> ELPQMTQQLNSDDMQEQLSATVKFRQILSREHRPPIDVVIQAGVVPRLVEFMRENQPEMLQLEAAWALTNIASGTSAQTKVVVDADAVPLFIQLLYTGSVEVKEQAIWALGNVAGDSTDYRDYVLQCNAMEPILGLFNSNKPSLIRTATWTLSNLCRGKKPQPDWSVVSQALPTLAKLIYSMDTETLVDACWAISYLSDGPQEAIQAVIDVRIPKRLVELLSHESTLVQTPALRAVGNIVTGNDLQTQVVINAGVLPALRL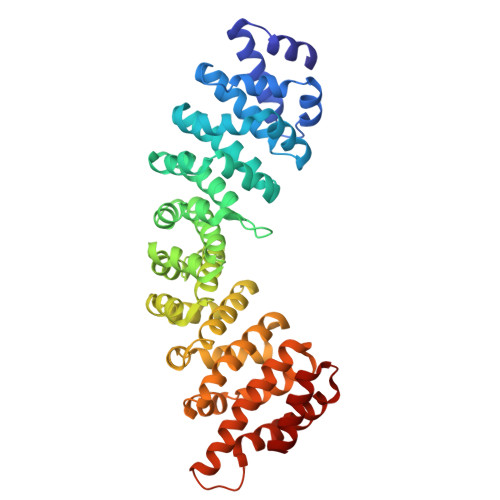LLSSPKENIKKEACWTISNITAGNTEQIQAVIDANLIPPLVKLLEVAEYKTKKEACWAISNASSGGLQRPDIIRYLVSQGCIKPLCDLLEIADNRIIEVTLDALENILKMGEADKEARGLNINENADFIEKAGGMEKIFNCQQNENDKIYEKAYKIIETYF>[3x]GSSHVTLPFYPKSPQSKDLIKEAILDNDFMKNLELSQIQEIVDCMYPVEYGKDSCIIKEGDVGSLVYVMEDGKVEVTKEGVKLCTMGPGKVFGELAILYNCTRTATVKTLVNVKLWAIDRQCFQTIMMRTGLIKHTEYMEFLKSVPTFQSLPEEILSKLADVLEETHYENGEYIIRQGARGDTFFIISKGTVNVTREDSPSEDPVFLRTLGKGDWFGEKALQGEDVRT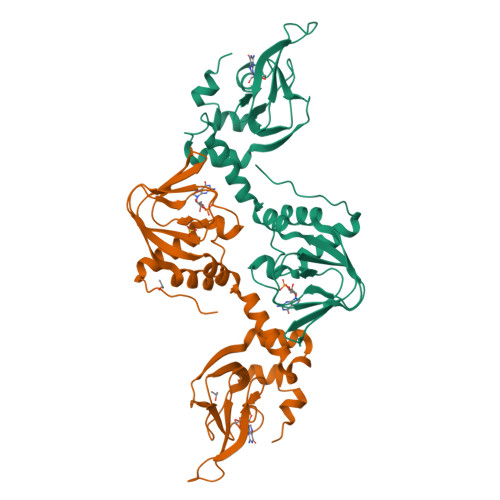ANVIAAEAVTCLVIDRDSFKHLIGGLDDVSNKAY>MAEMATATRLLGWRVASWRLRPPLAGFVSQRAHSLLPVDDAINGLSEEQRQLRQTMAKFLQEHLAPKAQEIDRSNEFKNLREFWKQLGNLGVLGITAPVQYGGSGLGYLEHVLVMEEISRASGAVGLSYGAHSNLCINQLVRNGNEAQKEKYLPKLISGEYIGALAMSEPNAGSDVVSMKLKAEKKGNHYILNGNKFWITNGPDADVLIVYAKTDLAAVPASRGITAFIVEKGMPGFSTSKKLDKLGMRGSNTCELIFEDCKIPAANILGHENKGVYVLMSGLDLARLVLAGGPLGLMQAVLDHTIPYLHVREAFGQKIGHFQLMQGKMADMYTRLMACRQYVYNVAKACDEGHCTAKDCAGVILYSAECATQVALDGIQCFGGNGYINDFPMGRFLRDAKLYEIGAGTSEVRRLVIGRAFNADFH[4x]

Isovaleryl-CoA (coenzyme A) dehydrogenase (IVD) is an intramitochondrial flavoenzyme that catalyzes the conversion of isovaleryl-CoA (3-methylbutyryl-CoA) into 3-methylcrotonyl-CoA in the leucine catabolism pathway, transferring electrons to the electron-transferring flavoprotein (ETF). Consistent with other ACADs, including short-, medium-, and long-chain ACADs, IVD is characterized by a tetrameric architecture composed of 4 identical subunits. Each subunit of IVD contains one noncovalently attached FAD molecule, imparting a characteristic yellow color to the purified enzyme. Dysfunction of IVD is linked to isovaleric acidemia (IVA), a rare metabolic disorder characterized by the accumulation of toxic metabolites.

To elucidate the complex structure with its substrates, an IVD construct with the E286A mutation was expressed and purified for cryo-EM preparation to minimize conformational instability caused by the process of enzymatic reaction. Thus, a mutant on the active site, E286A, was constructed and exhibited a stable combination with isovaleryl-CoA and butyryl-CoA, with apparent dissociation constant (KDapp) of 848 and 494 nM measured by surface plasmon resonance (SPR), which was utilized for cryo-EM sampling. Upon incubation with isovaleryl-CoA and butyryl-CoA, complexes of IVD with both substrates were resolved at resolutions of 3.35 and 2.91 Å, respectively. Following the addition of the 2 acyl-CoAs, the refinement process revealed additional tubular densities in the active site that ran partially parallel to the riboflavin portion of FAD, which were well-modeled as isovaleryl- and butyryl-CoA. The residues surrounding the active site create a relatively hydrophobic environment, facilitating the binding of both acyl-CoAs in a similar orientation. The residues involved in binding with 2 acyl-CoAs are predominantly identical. D284 and M280 form hydrogen bond interactions with adenosine at N6, while S222 and R223 contribute to interactions with the 3′-phosphate. In comparison, the activity of IVD for butyryl-CoA, which lacks a branched group, is no more than 30% of that for its optimal substrate. Comparison of the 2 acyl-CoAs in terms of binding revealed that butyryl-CoA exhibits a twist alternation in the fatty acyl portion, resulting in a longer distance and a less favorable angle between E286 and the Cα–Cβ bond of the substrate, which may contribute to its markedly lower catalytic efficiency compared to isovaleryl-CoA.PROPANOIC 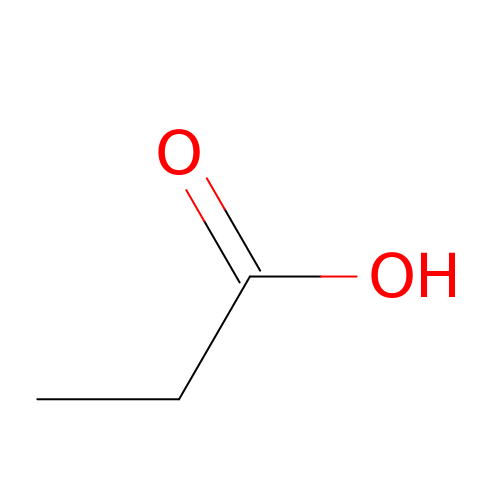ACID | C3 H6 O2 | XBDQKXXYIPTUBI-UHFFFAOYSA-N>MTVEPFRNEPIETFQTEEARRAMREALRRVREEFGRHYPLYIGGEWVDTKERMVSLNPSAPSEVVGTTAKAGKAEAEAALEAAWKAFKTWKDWPQEDRSRLLLKAAALMRRRKRELEATLVYEVGKNWVEASADVAEAIDFIEYYARAALRYRYPAVEVVPYPGEDNESFYVPLGAGVVIAPWNFPVAIFTGMIVGPVAVGNTVIAKPAEDAVVVGAKVFEIFHEAGFPPG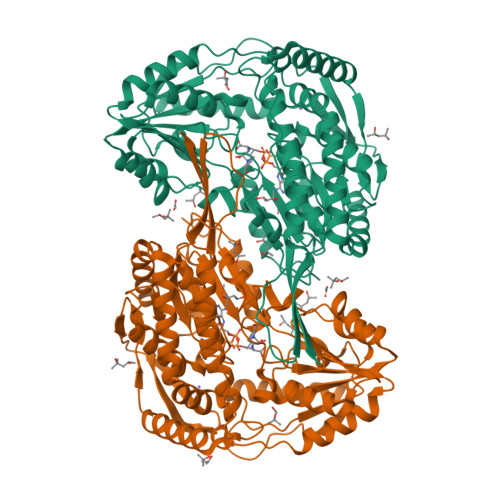VVNFLPGVGEEVGAYLVEHPRIRFINFTGSLEVGLKIYEAAGRLAPGQTWFKRAYVETGGKDAIIVDETADFDLAAEGVVVSAYGFQGQKCSAASRLILTQGAYEPVLERVLKRAERLSVGPAEENPDLGPVVSAEQERKVLSYIEIGKNEGQLVLGGKRLEGEGYFIAPTVFTEVPPKARIAQEEIFGPVLSVIRVKDFAEALEVANDTPYGLTGGVYSRKREHLEWARREFHVGNLYFNRKITGALVGVQPFGGFKLSGTNAKTGALDYLRLFLEMKAVAERF[2x]>[2x]MSLKRKNIALIPAAGIGVRFGADKPKQYVEIGSKTVLEHVLGIFERHEAVDLTVVVVSPEDTFADKVQTAFPQVRVWKNGGQTR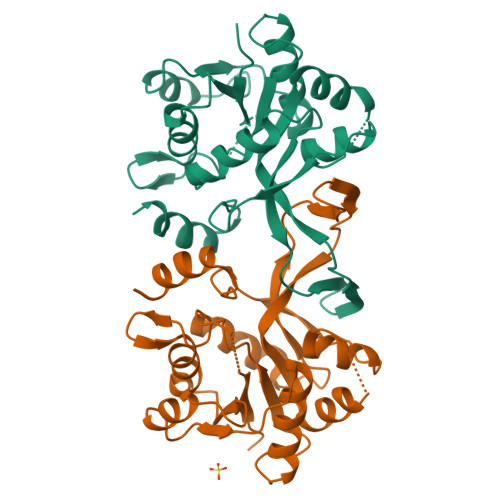AETVRNGVAKLLETGLAAETDNILVHDAARCCLPSEALARLIEQAGNAAEGGILAVPVADTLKRAESGQISATVDRSGLWQAQTPQLFQAGLLHRALAAENLGGITDEASAVEKLGVRPLLIQGDARNLKLTQPQDAYIVRLLLDAVEGGSHHHHHH> MEVTVPDALKDRIALKKTARQLNIVYFLGSDTEPVPDYERRLSELLLYLQQFYGKEMQRHGYGARSFGLDIKSPGRVNIIEYKAKNPAAHYPYENGGGWKAAQELDEFFKAHPDRKKSQHTLIIMPTWNDEKNGPDNPGGVPFYGMGRNCFALDYPAFDIKHLGQKTREGRLLTKWYGGMAAALGHGLNLPHNHQTASDGKKYGTALMGSGNYTFGTSPTFLTPASCALLDACEVFSVTPSQQFYEGKPE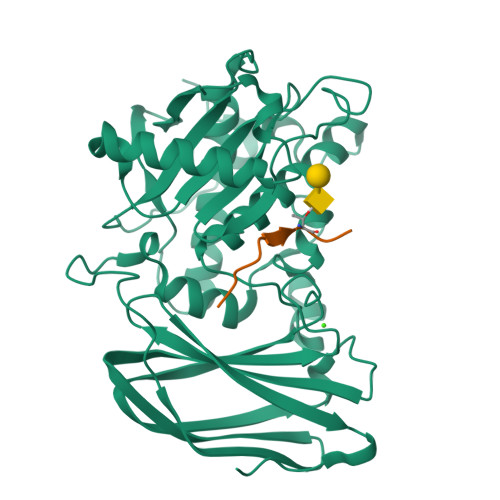VEVGDVAISFKGDQILVSGNYKSPQTVKALNVYIQDPPYAVNQDYDAVSFSRRLGKKSGKFSMKIDKKELEGLNNNEFRISLMFILANGLHMQKHFTFHWDALQDYRDGSKSGSGHHHHHH;> GKPRPYSPRPTSHPRPIRV> SVRD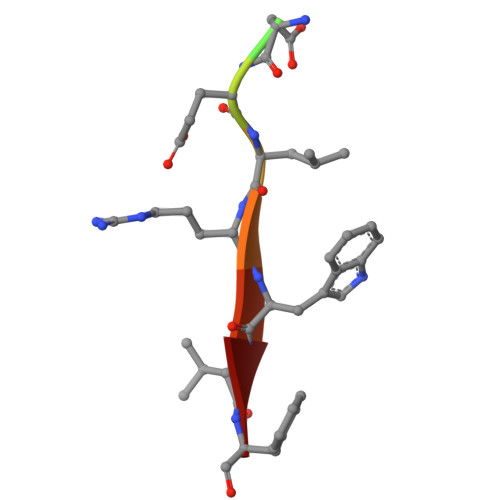ELRWVF> GLEKTVKEKLSFEGVGIHTGEYSKLIIHPEKEGTGIRFFKNGVYIPARHEFVVHTNHSTDLGFKGQRIKTVEHILSVLHLLEITNVTIEVIGNEIPILDGSGWEFYEAIRKNILNQNREIDYFVVEEPIIVEDEGRLIKAEPSDTLEVTYEGEFKNFLGRQKFTFVEGNEEEIVLARTFAFDWEIEHIKKVGLGKGGSLKNTLVLGKDKVYNPEGLRYENEPVRHKVF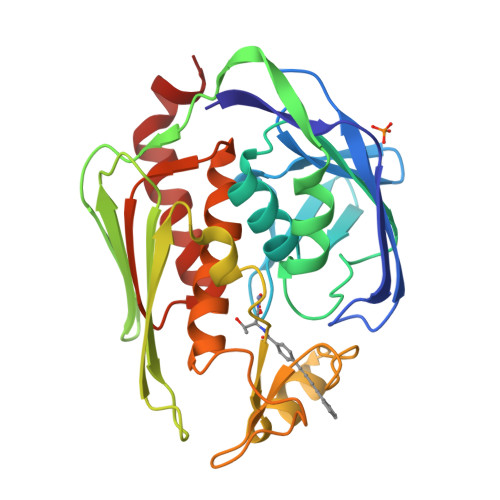DLIGDLYLLGSPVKGKFYSFRGGHSLNVKLVKELAKKQKLTRDLPH(3S,6R)-6-[(3R,5R,8R,9S,10S,13R,14S,17R)-10,13-dimethyl-3-(2-methyl-2-oxidanyl-propyl)-2,3,4,5,6,7,8,9,11,12,14,15,16,17-tetradecahydro-1H-cyclopenta[a]phenanthren-17-yl]heptane-1,3-diol 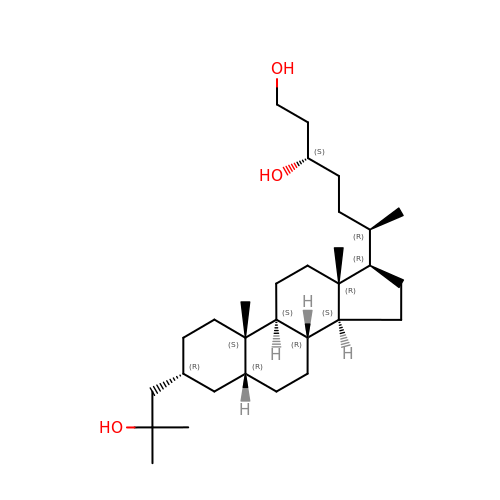| C30 H54 O3 | BELGEHMGZKEZEK-XXWWFROJSA-N>MRGSHHHHHHGSMQILLANPRGFCAGVDRAISIVENALAIYGAPIYVRHEVVHNRYVVDSLRERGAIFIEQISEVPDGAILIFSAHGVSQAVRNEAKSRDLTVFDATCPLVTKVHMEVARASRRGEESILIGHAGHPEVEGTMGQYSNPEGGMYLVESPDDVWKLTVKNEEKLSFMTQCTLSVDDTSDVIDALRKRFPKIVGPRKDDICYATTNRQEAVRALAEQAEVVLVVGSKNSSNSNRLAELAQRMGKRAFLIDDAKDIQEEWVKEVKCVGVTAGASAPDILVQNVVARLQQLGGGEAIPLEGREENIVFEVP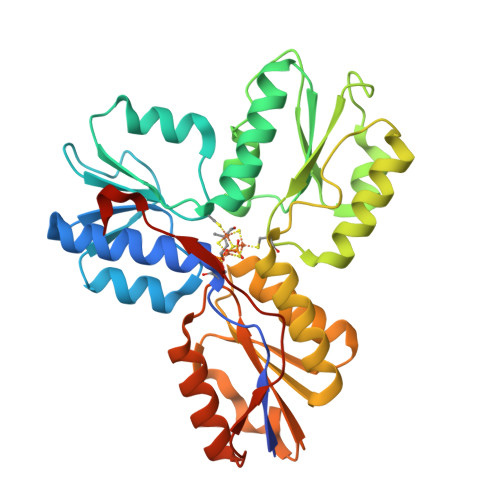KELRVDIREVD[2x]> MYVFRFHISSFHSFLVNFLQPSRGVGEPSRLLHHLETHPSYMRRVTSTAVHRTVSSVLSPALLPSFNGTLLLSVCFASCSAAPVRNLYKRLGLDHKATSEEVKAAYRQRAL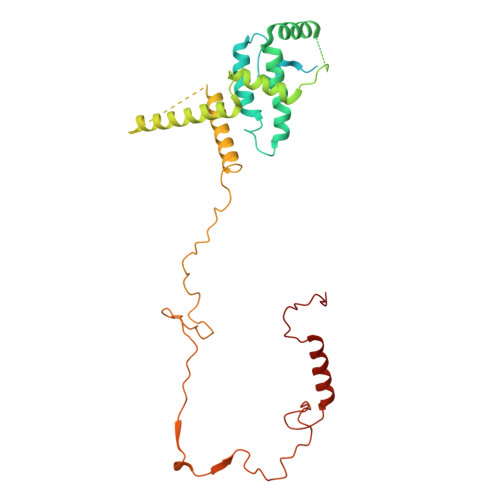ECHPDVVDDNQKAQAEVDFRAVSEAYDVLIDPQKRKEHDKALGLERTVPPAKKQQEGEGVGCDSKGSFNRGVTRPRNRKPFVRGDADRNFREAFHGMSLDQVLFRERLRQRRMQKQMEEKAKSSSSSSSSSSSSSSSSSSSSSSSSSSSSSSSSSSSSSSSSSSSSSSSSRDPQPPPSDYMPFRPFHGWTVPNGVRTPPEPTLGPTAKVEDVKDVQLAEPAVGDASHQRKLPKHFPVVQASDGSSLLREETIACMERERRLPHNMGKLYSYHRPY> SNAMFAPQGLAQFIKVNVTLENGEPVFIYTDANGQVCQGDITVTQAGTITYLLNDQTLKGLKFVGVGFVTPFDGIIDAVTIS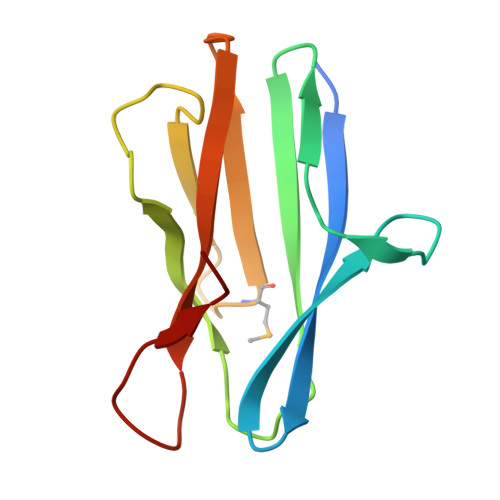SDGMLVQLVDLDKTPGTTKFQFVLSNTANTLLVLSPD> EDIKVAVVGAMSGPVAQYGDQEFTGAEQAVADINAKGGIKGNKLQIAKYDDACDPKQAVAVANKVVNDGIKYVIGHLCSSSTQPASDIYEDEGILMITPAATAPELTARGYQLILRTTGLDSDQGPTAAKYILEKVKPQRIAIVHDKQQYGEGLARAVQDGLKKGNANV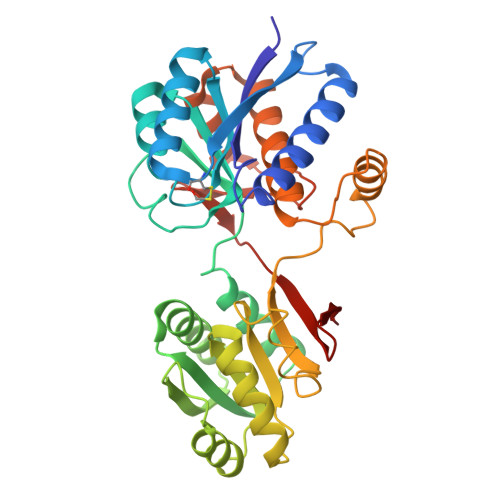VFFDGITAGEKDFSTLVARLKKENIDFVYYGGYHPEMGQILRQARAAGLKTQFMGPEGVANVSLSNIAGESAEGLLVTKPKNYDQVPANKPIVDAIKAKKQDPSGAFVWTTYAALQSLQAGLNQSDDPAEIAKYLKANSVDTVMGPLTWDEKGDLKGFEFGVFDWHANGTATDAK> AIKSSILSFNSIITKNDEIKNEEAEFPKVLLFNDNYFDGNIYRINNALSGIEHDPMYYDLMCQSMKQQIEKIKIPLNSSETISVFAIAPQPLLLYLGYLLNDETNIKIYQRFRTGNLKWNWESSEITNNFYVEQLYTDGNEIDTEVNLILSLSAEISLDRIPTFSNQEYKVPTLILRSDRQGFDAIKSNEDVNEYISVFRNLVVEKIRNDFPNLKCINIFPATPVSVPVRMGMNYQKN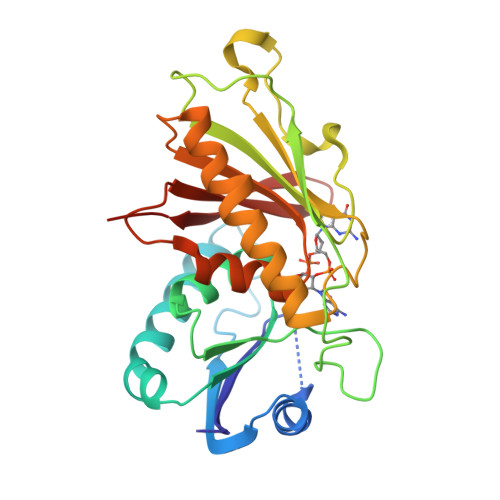IDVEWKIFNQQTNVGFIYSLSLKGEV>MSEKKEARVVINDLLAEQYANAFKAKEEGRPVGWSTSVFPQELAEVFDLNVLYPENQAAGVAAKKGSLELCEIAESKGYSIDLCAYARTNFGLLENGGCEALDMPAPDFLLCCNNICNQVIKWYENISRELDIPLIMIDTTFNNEDEVTQSRIDYIKAQFEEAIKQLEIISGKKFDPKKFEEVMKISAENGRLWKYSMSLPADSSPSPMNGFDLFTYMAVIVCARGKKETTEAFKLLIEELEDNMKTGKSSFRGEEKYRIMMEGIPCWPYIGYKMKTLAKFGVNMTGSVYPHAWALQYEVNDLDGMAVAYSTMFNNVNLDRMTKYRVDSLVEGKCDGAFYHMNRSCKLMSLIQYEMQRRAAEETGLPYAGFDGDQADPRAFTNAQFETRIQGLVEVMEERKKLNRGEI[2x];>MEAILSKMKEVVENPNAAVKKYKSETGKKAIGCFPVYCPEEIIHAAGMLPVGIWGGQTELDLAKQYFPAFACSIMQSCLEYGLKGAYDELSGVIIPGMCDTLICLGQNWKSAVPHIKYISLVHPQNRKLEAGVKYLISEYKGVKRELEEICGYEIEEAKIHESIEVYNEHRK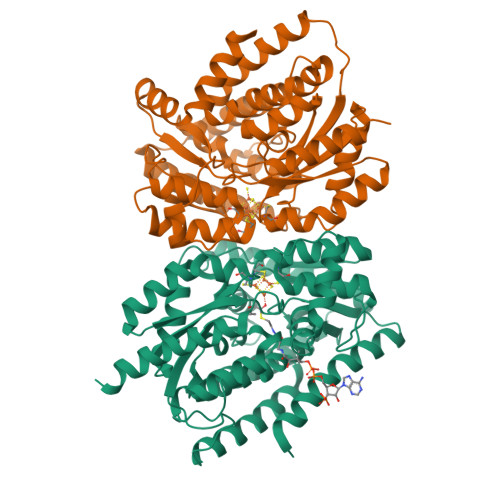TMRDFVEVAYKHSNTIKPSIRSLVIKSGFFMRKEEHTELVKDLIAKLNAMPEEVCSGKKVLLTGILADSKDILDILEDNNISVVADDLAQETRQFRTDVPAGDDALERLARQWSNIEGCSLAYDPKKKRGSLIVDEVKKKDIDGVIFCMMKFCDPEEYDYPLVRKDIEDSGIPTLYVEIDQQTQNNEQARTRIQTFAEMMSLASAWSHPQFEK[2x]>MVQKESQATLEERESELSSNPAASAGASLEPPAAPAPGEDNPAGAGGAAVAGAAGGARRFLCGVVEGFYGRPWVMEQRKELFRRLQKWELNTYLYAPKDDYKHRMFWREMYSVEEAEQLMTLISAAREYEIEFIYAISPGLDITFSNPKEVSTLKRKLDQVSQFGCRSFALLFDDIDHNMCAADKEVFSSFAHAQVSITNEIYQYLGEPETFLFCPTEYCGTFCYPNVSQSPYLRTVGEKLLPGIEVLWTGPKVVSKEIPVESIEEVSKIIKRAPVIWDNIHANDYDQKRLFLGPYKGRSTELIPRLKGVLTNPNCEFEANYVAIHTLATWYKSNMNGVRKDVVMTDSEDSTVSIQIKLENEGSDEDIETDVLYSPQMALKLALTEWLQEFGVPHQYSSRQVAHSGAKASVVDGTPLVAAPSLNATTVVTTVYQEPIMSQGAALSGEPTTLTKEEEKKQPDEEPMDMVVEKQEETDHKNDNQILSEIVEAKMAEELKPMDTDKESIAESKSPEMSMQEDCISDIAPMQTDEQTNKEQFVPGPNEKPLYTAEPVTLEDLQLLADLFYLPYEHGPKGAQMLREFQWLRANSSVVSVNCKGKDSEKIEEWRSRAAKFEEMCGLVMGMFTRLSNCANRTILYDMYSYVWDIKSIMSMVKSFVQWLGCRSHSSAQFLIGDQEPWAFRGGLAGEFQRLLPIDGANDLFFQPPPLTPTSKVYTIRPYFPKDEASVYKICREMYDDGVGLPFQSQPDLIGDKLVGGLLSLSLDYCFVLEDEDGICGYALGTVDVTPFIKKCKISWIPFMQEKYTKPNGDKELSEAEKIMLSFHEEQEVLPETFLANFPSLIKMDIHKKVTDPSVAKSMMACLLSSLKANGSRGAFCEVRPDDKRILEFYSKLGCFEIAKMEGFPKDVVILGRSL[2x]

Human O-linked β-N-acetylglucosaminidase (hOGA) is one of the two enzymes involved in nuclear and cytoplasmic protein O-GlcNAcylation, an essential post-translational modification. The enzyme catalyzes the hydrolysis of the GlcNAc-O-(Ser/Thr) glycosidic bonds via anchimeric assistance through the 2-acetamido group of the GlcNAc sugar. OGA is a multidomain enzyme comprising a nonfunctional acetyltransferase domain, a glycoside hydrolase domain that belongs to CAZy family 84 (GH84), and a structurally important stalk domain involved in dimerization. GH84 enzymes operate via anchimeric assistance by the 2-acetamido group of the GlcNAc sugar of the substrate.15−20 The reaction mechanism involves two distinct chemical steps (named “cyclization” and “ring opening”, respectively), leading to hydrolysis with retention of configuration at the anomeric center.

Here we report a crystal structure of wild type hOGA in complex with a nonhydrolyzable glycopeptide substrate in which the peptide is S-GlcNAcylated at a cysteine residue. Crystals of WT hOGA, protein produced by coexpression of the glycoside hydrolase domain (residues 11–396) and the stalk domain (535–715),11 were seeded with a known peptide substrate derived from casein kinase II (CKII) (339-YPGGSTPVSSANMM-352) and the corresponding CKII-Cys-GlcNAc glycopeptide. This peptide was produced by S-GlcNAcylation using OGT. Crystals of WT hOGA and the CKII-Cys-GlcNAc complex diffracted to a resolution of 2.5 Å. The resulting hOGA-CKII-Cys-GlcNAc structure shows density at the active site, corresponding to GlcNAc-Cys. GlcNAc was bound in a 1,4B/1S3 conformation, with several interactions between the GlcNAc moiety and hOGA residues, from N2, O7, O3, O4, and O6 of GlcNAc, to D174, N280, K98, G67, N313, and D285 that have been previously characterized.11 The peptide could be partially built into the active site of one monomer. Surprisingly, only two of the 14 residues of the peptide could be modeled, Cys347 and Ser348, and no interactions were observed between the CKII peptide and the active site residues of hOGA. Such weak interactions between the CKII peptide and hOGA could allow for flexibility and accommodation of the vast range of known protein targets within the active site. In summary, the results of both X-ray crystallography and QM/MM simulations reported are consistent with hOGA using a preactivated 1,4B/1S3 conformation for catalysis.>[3x]SPAGVLVDAMSQKHLQINQRFEELRLITQDTENELKKLQQTQEYFIIQYQESLRIQAQFAQLGQLNPQERMSRETALQQKQVSLETWLQREAQTLQQYRVELAEKHQKTLQLLRKQQTIILDDELIQWKRRQQLAGNGGPPEGSLDVLQSWCEKLAEIIWQNRQQIRRAEHLCQQLPIPGPVEEMLAEVNATITDIISALVTSTFIIEKQPPQVLKTQTKFAATVRLLVGGKLNVHMNPPQVKATIISEQQAKSLLKNENTRNECSGEILNNC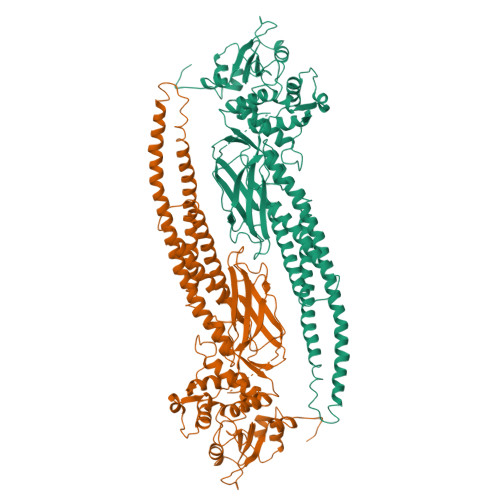CVMEYHQATGTLSAHFRNMSLKRIKRADRRGAESVTEEKFTVLFESQFSVGSNELVFQVKTLSLPVVVIVHGSQDHNATATVLWDNAFAEPGRVPFAVPDKVLWPQLCEALNMKFKAEVQSNRGLTKENLVFLAQKLFNISSNHLEDYNSMSVSWSQFNRENLPGWNYTFWQWFDGVMEVLKKHHKPHWNDGAILGFVNKQQAHDLLINKPDGTFLLRFSDSEIGGITIAWKFDSPDRNLWNLKPFTTRDFSIRSLADRLGDLNYLIYVFPDRPKDEVFAKYYTPVLAKAVDGYVKPQIKQVVPEFVNASTD>GSHMEYCPKMLSEIRQEDINDVETVAYVTVTGKTARSYNLQYWRLYDVPKTAPSQWPSFGTLRDDCGNIQLTA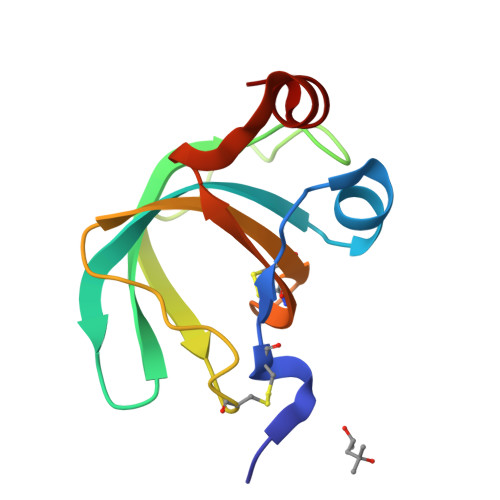DTDYVLGCKSGNQDCFVKLHDGLSQKEKDLLKE[7x]DEOXYURIDINE-5'-TRIPHOSPHATE | C9 H15 N2 O14 P3 | 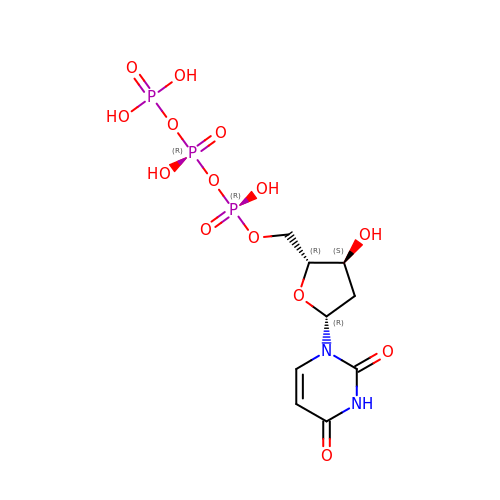AHCYMLUZIRLXAA-SHYZEUOFSA-N>[6x]MKTIFSGIQPSGVITIGNYIGALRQFVELQHEYNCYFCIVDQHAITVWQDPHELRQNIRRLAALYLAVGIDPTQATLFIQSEVPAHAQAAWMLQCIVYIGELERMTQFKEKSAGKEAVSAGLLTYPPLMAADILLYNTDIVPVGEDQKQHIELTRDLAERFNKRYGELFTIPEARIPKVGARIMSLVDPTKKMSKSDPNPKAYITLL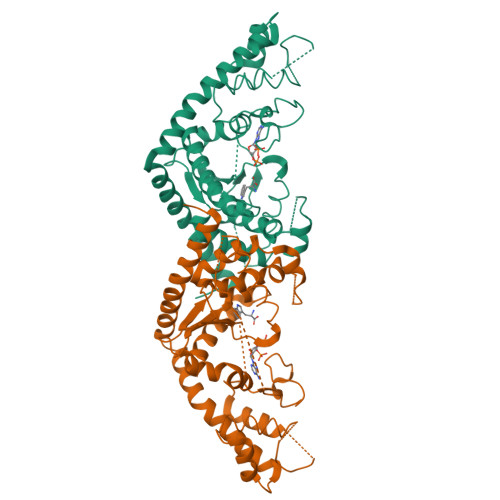DDAKTIEKKIKSAVTDSEGTIRYDKEAKPGISNLLNIYSTLSGQSIEELERQYEGKGYGVFKADLAQVVIETLRPIQERYHHWMESEELDRVLDEGAEKANRVASEMVRKMEQAMGLGRRR> SDSLSKSPENWMSKLDDGKHLTEINIPGSHDSGSFTLKDPVKSVWAKTQDKDYLTQMKSGVRFFDIRGRASADNMISVHHGMVYLHHELGKFLDDAKYYLSAYPNETIVMSMKKDYDSDSKVTKTFEEIFREYYYNNPQYQNLFYTGSNANPTLKETKGKIVLFNRMGGTYIKSGY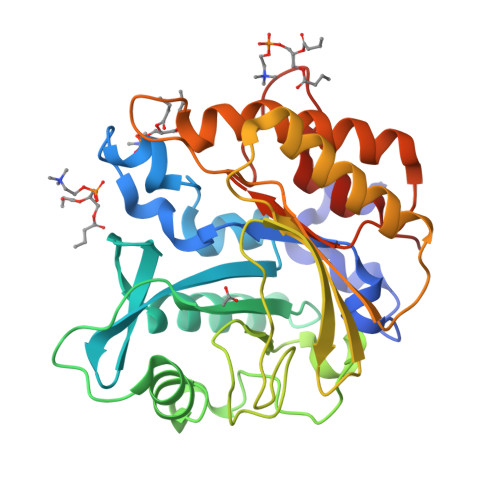GADTSGIQWADNATFETKINNGSLNLKVQDEYKDYYDKKVEAVKNLLAKAKTDSNKDNVYVNFLSVASGGSAFNSTYYYASYINPEIAKTIKANGKARTGWLIVDYAGYTWPGYDDIVSEIIDSNKLEHHHHHH>AEEFPVPNGFESAYREVDGVKLHYVKGGQGPLVMLVHGFGQTWYEWHQLMPELAKRFTVIAPDLPGLGQSEPPKTGYSGEQVAVYLHKLARQFSPDRPFDLVAHDIGIWNTYPMVVKNQADIARLVYMEAPIPDARIYRFPAFTAQGESLVWHFSFFAADDRLAETLIAGKERFFLEHFIKSAASNTEVFSERLLDLYARSYAKPHS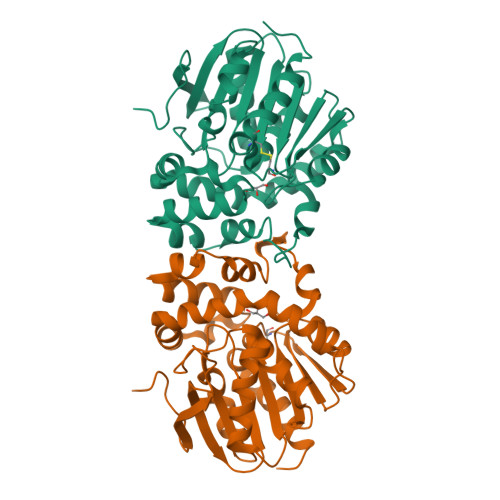LNASFEYYRALNESVRQNAELAKTRLQMPTMTLAGGGHGGMGTFQLEQMKAYAEDVEGHVLPGCGHWLPEECAAPMNRLVIDFLSRGRHHHHHH[4x]> MAISLATKAATDALKVNRAPVGVEPQEVHKWLQSFNWDFKENRTKYATKYHMANQTKEQFKVIAKEYARMEAAKDERQFGTLLDGLTRLGAGNKVHPRWGETMKVISNFLEVGEYNAIAASAMLWDSATAAEQKNGYLAQVLDEIRHTHQCAFINHYYSKHYHDPAGHNDARRTRAIGPL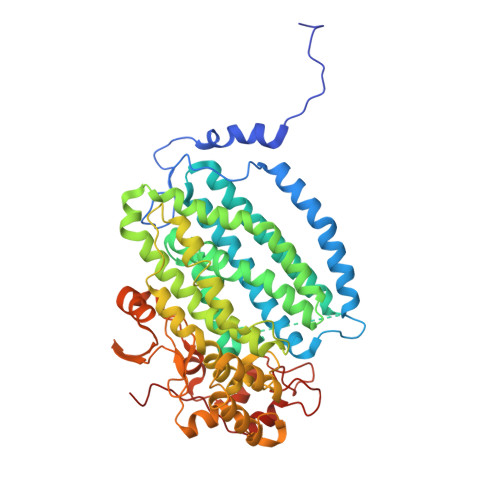WKGMKRVFADGFISGDAVECSVNLQLVGEACFTNPLIVAVTEWASANGDEITPTVFLSVETDELRHMANGYQTVVSIANDPAAAKYLNTDLNNAFWTQQKYFTPALGYLFEYGSKFKVEPWVKTWNRWVYEDWGGIWIGRLGKYGVESPRSLRDAKTDAYWAHHDLALAAYALWPLGFARLALPDEEDQEWFEANYPGWADHYGKIYNEWKKLGYEDPKSGFIPYAWLLANGHDVYIDRVSQVPFIPSLAKGSGSLRVHEFNGKKHSLTDDWGERMWLSEPERYECHNLFEQYEGRELSEVIAEGHGVRSDGKTLIAQPHVRGDNLWTLEDIKRAGCVFPNPLAKF> RVRKLPET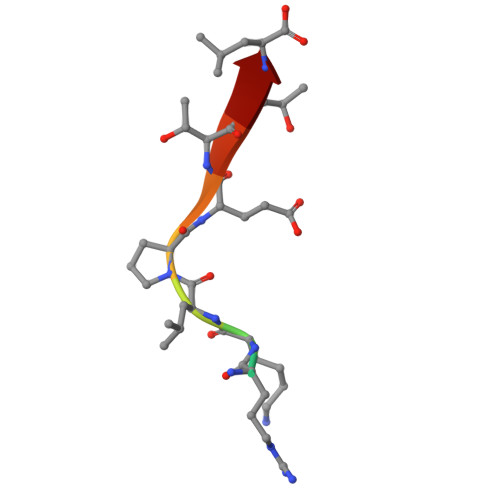TL> MINNKQIQKIQQISKFQLKEYIEMQMQQHSLNKQIKEEERNYILLENAIDNSNIQGFQTIQEIVQLAMQRM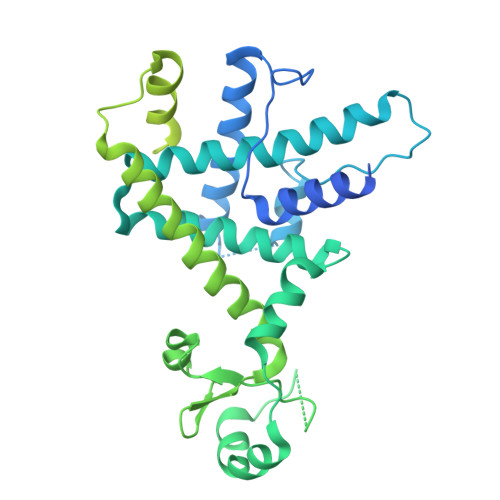KMIKEIIQEEPRFNLIDPLSKPNYNRIRVANKFITVAIPKSDPEYELKNKQQYAKEVLSHFLCKMAYAFYAEPETWLEFARAEAFILMDKLKSGQHHANFFSDENLKIKTISDELFKQAFPKIEATFSSIKIKKNDSEVEQINIKKDNFKMFKFIDHPSMLSNNDVVLHKGYIIIYKESTSKIVQNIFIERLLDEMRLLQLKFQNNGSKLDDDRLSFLKDLHKAEIFNDSTQFNSTQIHHYELDRLAKRDMPACMTYLMYGLNQKLHLKHFGRLQLGLFLKGAGLSLNEALTFWQKKFSKTSADDFKKKYDYNIRHNYGKLGKQLDYTPMSCQKIIGFQPLKDEFHGCPYKTMESQQLKDFLKLSYNITDEQFVQVNIFKNQKQYQLACKEVFKVLNDTRDKTKEQFYPYFDKVGNHPNAYFEQSLRMHEPQRFQKQDEEKKQNKQNRNQNFSANKQSTNKNNQMDLEF> VDSTELTPSEAQSAIDDINAAVETLKEIQSEEPKADWSKEFDKLFATATELTQSLAVVAGGYQTLANPDLIMARTHLIVEIGLTVDKSANNLRYKIQKAHVELGFSVTRAIMRVANIGATVYQLNDSISDLRATYERVSTYRDLK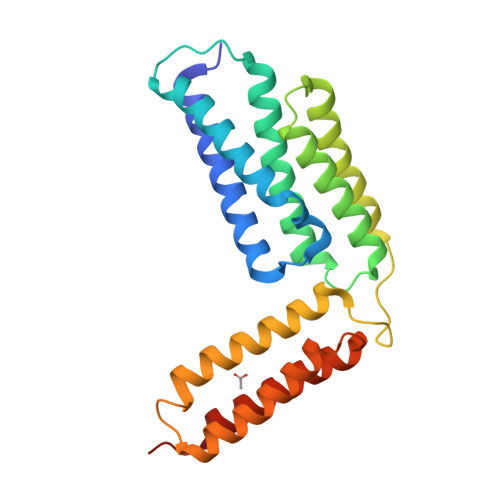STDTATIYVKDLLNKAIWNTRVARDKEILTHKNFRTYQTLNKEITKAVRVWFKAKATVAECDAAIAKLNTAYATAYSAPSVRAAAS(5M)-5-(2-methoxyphenyl)-1,3,4-oxadiazol-2-amine | C9 H9 N3 O2 | 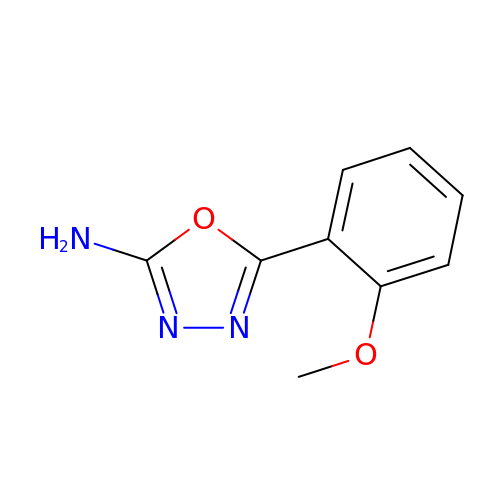HTILGWBWTPTFES-UHFFFAOYSA-N>MDLTINYKSTLGDDVAAYIYKETNKPAGEWPGKTMTATAGHEGWYTMHLTLDNSTDYSLILNDDGHGNQLKDVTLSTKGKAEAEYWFDGSLSETKPA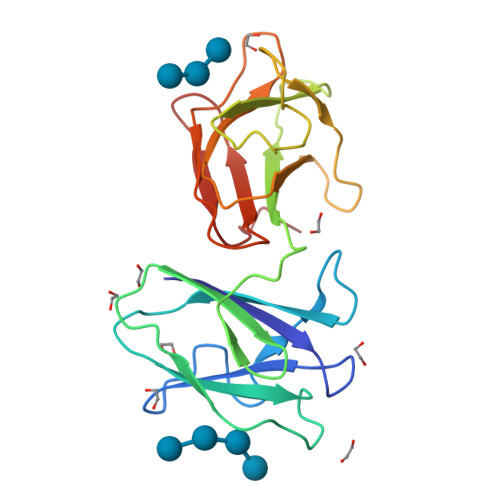DWKYVTTIHYLASGMGSTIYNYMWGADASATGAGVGKEWPGGQISANADHLGWYDVVYTQDVKQNFSCIFNNNNGTQTDNIDVSVTSTSTELWVTGTKGDTTVYKTAPDSWE[2x]> MTEHRSVRFSAPRPSWRPAGDDTPLAGLECATVTVPVDHARPDGPTLEVALARHPARSAGRRRGVLLVGPDDPGNPGTLLVPQLVRDLPADVLD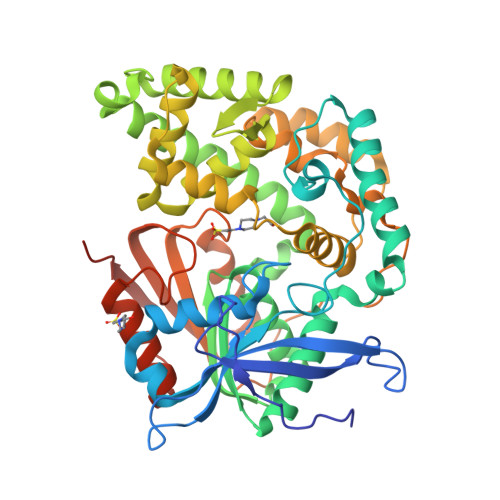GYDVVGFDHRFSGGSAPLSCGLTPDQWLWIFHRPQDVESEARFQRAVVERCFDAAGDVLPYLTSRDIARDMDVIRRALGEDRISYLGHSYGSYLGAVWTQMFGEHADRVVLDSVIDPSSVWRRMFLDYAVSCEAALERWAHWAAERDGELDLGRDAPTVRAALDALAGRADREPLPVAGMPVDGTMLRLFTMVLLSSDRAWGFLGDIVRAAVHGDEAAPSTLRALGAMFGRGKEESGAVAQLGVLCGDAAWPRDMEVYRRDLAGHGARHPFIGPAMAGPKAGAFWPVPPAEPVTVLGADNRAESVLLVQSEQDMFTPARGARRMRELLAHNTRLVTLAGAVQHRVFPFHGDPGVNRAAAAYLLTGKLPDTDLTLRAAAADGGPAGEGSPS> DPKLNFSWPVNVGPLNPHLYSPNQMFAQNMVYEPLVHYNADGTVGPWLAESWEASQDGRSYTFKLREDVKFSNGEVFDAAAVKANIDTVLQNRPRHNWLELVNQMVSAEVVGPYKVRINLKKPYYPLLQELSLPRPFRFIAPSQFKNGGTADGIVAPIGTGPWKLTETKLGEHDVFTRNDSYWGPKPAYEQITVKVIPDPNTRAIAFEAGEIDLIYGTEGPISPDTFERFQKMGIYNTELSEPLETRVLALNTNHGATKDLAVRKAINHAVDKDTMIATVLYGTQKRADTLFADNVPYANIGLKPYAFDPALAARLLDEAGWTAKASGDIREKDGQPLAIELCFIGTDAISKSMAEIVQADLRKVGIDVKLTGEEESSIYARQRDGRFDMIFNQTWGAPYDPHAFVSSMRVPSHADYQAQLGLPDKAKIDAEIGQVLVSTDETARQALYKDILTRLHEEAVYLPLTSVTAMAVAKPEV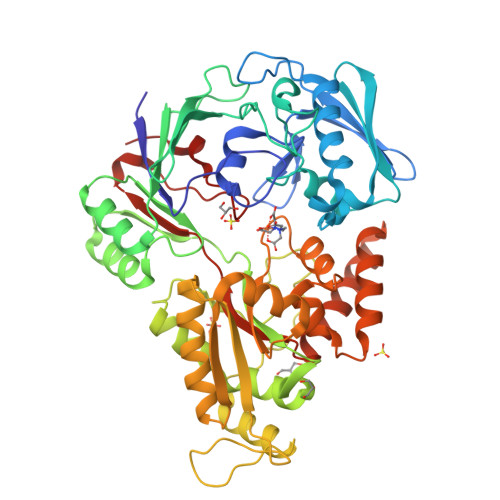GKITFGAMSSEIPFEKLTPKAN> MWHYTSINNDTRVALDPKPNQIRTITKPNTVPQLGTDYLYTFNSQRRSHTLRLLGPFQYFNFSETDRGHPLFRLPLKYPSKAIPADELIDNLHSWMRSVHLLHVRSEDNTLRYNWMLGVYARSTNYTTPVGQLVVNAPAILNYSNPQDAFNSVFVALGIDYIDIPITNSNIFDDSSTPYNVRIWHAPTMTEVNHILALMRKSTLVSTHSSWHWNVLHTFHYRSESDMIDHFAAKILEDWRQKEKLDKGALVEADRVIQRLIPLSSSTYVQRLAAIGALYPNEFTENVLDLSRLSTALLQLSDTYYQHANDQLRRLYRRMYNDSRTLYMTQRHQELLLAQITADPNILLYPYTYIFTTIPTSMNYISNTGQGRIKHSLTVTGATEHDTVADIVLGQTGEDVITISMVEPMSIAVEDMYGYVLDTPTRDIWPADEQIEQKGDAVALYDTKTSRALGMFNNTVRIDDLLSPLLSLVYRTYIKGDTMTMTQGSLDHLTLCAAVDSDITFVG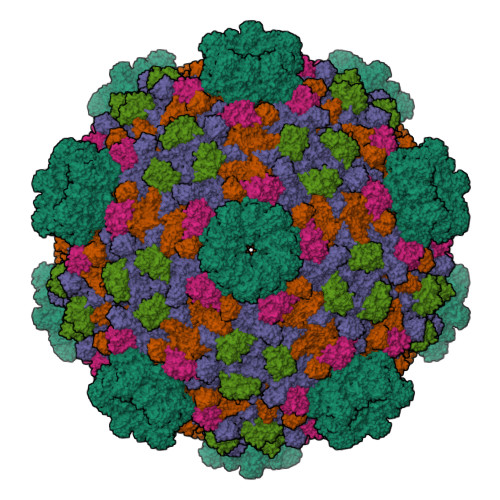NRMIAPLPEGYIPKPMHRNNSTMKMLSLYVALKKLENFATNSYLMAPDTSIILLGAEREPAVNILRRFNRNVSNVRIIGMGDRAVEPNIRVRVPFPIDKNISADFIICDINSYEDQSFESMFSETISVVTTCASAATRALVKINHPSEYMINSVIERLSQLGGVFYHTALLKTASQNPYSYETYIYITPIAAAVRFPFYSNSAMINRYMTAVADDEMPIIPSIHTVIKGHSNTYSPGLFCGCVDVQSAPLALSQLKSYCSEATTWRVDSDDNLVNIIARIDPARIALEFRTRSNTSAYHEYQRYVPNGLGFKVRKTREFRYMHREVTFIHKLMMYALIREQISLTENMTQVVSIGGRNLADISVVPLNMKYVVIDPATRIETLTQEKKNIEVQSRPFQFDAANMDLENNSIYLFIAVIMNEPNGAATPARMQMDKIRNVATAMLTRTNCVAYISFYEAGIITRLDQSTAHKTIRVEEGRLKVANYVPVDTLVEADVTLMLRDIGITHEIIRPSTPELIDACSNYGIRLGSTGGAVLDVFNHYSPVIKLVRS;>MHSTNNNSNKRNNEEKHKQPEIDSSANNGEGTSGTRAQTVGDTATEAGVRNETEAGASTRRQTDGTGLSGTNAKIATASSARQADVEKPADVTFTIENVDDVGIMQQKKPPTVVQSRTDVFNEQFANEALHPTTKVIFNGLDVNTEVQPLSDDFKQISDPKGYLTYSVKYEDQFTKKDKLRASEADDRIVGPTVNLFKYGAAVVNIDLNRDFFDTATGIDLTKGIPLVQDLLVPIGVTAGAEQSAEYVSGLLMVLFKVMTDNRLVIVGETTTPMSNTLSTVVNNVLRTTYHNNVGVNPALLRDFTQVNWLNRDITNMLQQAGTKYGLGLTETRLDYVRLVKTIVGHALNIDHFAASVLNINLRALMEANVTADDRIKALQAHSMISTQFHGPNQGALRPELAFDHDHIIRCLMLAAANYPRLEGIIVQINTGYVASANVIRPVSEKRYFPENLEQNQSAARLVSAVKARASEADISSIHLAIAREVSPMFNVHELKKIAESFEDPSSIVVVLEFILFALFFPTEFNRIKGDIQNVLLLFFSRWYPVEYGIFVQRGATYTINAAGEFEFSGRNEKWDQALYLSEHFPALFSDVPLAGANTIIAIMRLFTPQGFLRTDDLAIAANFPRASRNPQTYIPYTNQRGTVTNEFASRFRTIVATLANVVNERAVQDDMQKATRSCTKQWLRHLETQFDNIAVAHTDHLSVVYATMSNFMLNFTNNFSGNHATFKPDQYVITSPEGSYKPIIERQGETVDGLTIIDTSIVWPILCQCTYPLVRQSGKGVDAVSIMEEIVYPDPSTTLSQSLSVAQVLSKLTLPDAFINMILSGGDSVVMRTYQTEADDDLDEGIRMTTYDQYLSHIRERLHITNVPDPIYITGASTPDQIAASVQATHVAVVLYQSGVINGPASTYLRENEVLVVMPDYYDVVSRFANANLQMNNNRYHESVLEIADIFDQADFIQTSDAVRQLRALMPTLSTSQIRHAIERIAQITDVDSTDYGKLTLRFLGTLTRSLKMQNAQIRRIRPDGTVLRYDDQIDIEAFRWSRYFLDELQLRRLSVGLRLITNPRIARRFNGVRIMYLTDDDPDPDFVPDVPEGYVAVQYAHRLFSSSLANKRNRVTYTHPPTGMAYPSPTGRPHVHMTINERAGMSKLVADNIIASVIKSNWVVDILDIEYTAEVMTPSEGYTQHVDAESIMTAPKGKLFHLQFMDGLLRPEPSAFDPPASGEDMRLIYPLQPISVARSMRAIVNHNEVDRPRGAVAPSSYEMDTGTLSRNGDLLYSPVANGQVGIPKLEVDHISFSNVVSMMTANIRTGDDMAVERVNPDDVRAINIRNA[2x];>[2x]MLQQPTGGYTTLEQFAFTIRNDGTNATPTQFLQLLSYEATENELVKKTIPTPETHLPSARNVPGNVYIEDAITQALFGISAQNVNAHGYFSRLSALALPNTSARLGLDGVIYNSETINIPFYDPAAVANFAATYAKLGNASTPRYRADMIDIYAHVGLELAGTDAERAAGVMPVKRAKFDSWEGSLISLSRDVVNWKILAFLIDLCSLEGEALRAFKTRNRDVFRMMLFIMSTAVAANVVNRKVTKRVDRVLEYIGVNSMRTAGRTATITYDLSRHEFAAKFLQLTFTRWNAASAMIRSMPDMHTPRTSITPAGENALVRHNRYMTENFKGLSPIALAQKKHEMMLHTHEIHSMDIDGSIKNMVERETVNKMNEIDAMNTAPWTEEFAEVEPTTVYERHQIGTDPEQTQLISQDAAVIVHQASSDVDENEYGNSVSELTIDTQSDSVL> GEVANPEHYIKHPLQNRWALWFFKNDKSKTWQANLRLISKFDTVEDFWALYNHIQLSSNLMPGCDYSLFKDGIEPMWEDEK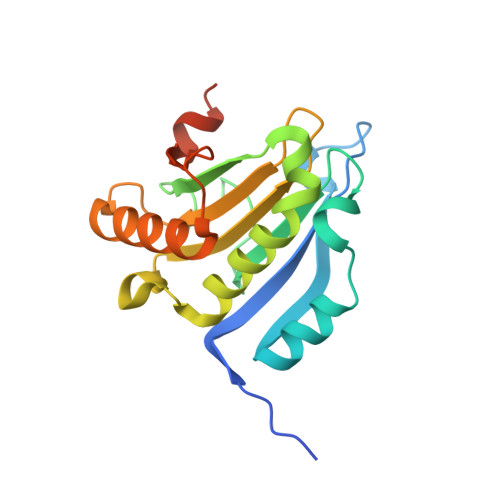NKRGGRWLITLNKQQRRSDLDRFWLETLLCLIGESFDDYSDDVCGAVVNVRAKGDKIAIWTTECENRDAVTHIGRVYKERLGLPPKIVIGYQSHADTATKSGSTTKNRFVV>[5x]NEAVKTLDGWFCLHDFRSIDWAAWRELNPGNQELMLNELSHFLSDMEIT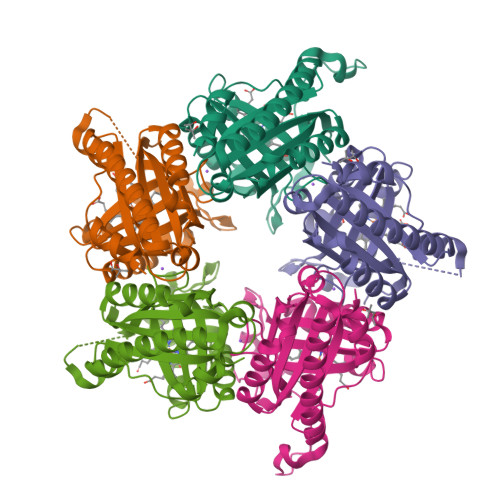KNIGEGEHTIYSILGQKADLVFFTLRDSLEALNEVENRFNKLAIADYLLPTYSYISVVELSNYLASHMAGGDDPYQNKGVRARLYPALPPKKHICFYPMSKKRDGADNWYMLPMEERQQLIRDHGLIGRSYAGKVQQIIGGSIGFDDYEWGVTLFSDDALEFKRIVTEMRFDEASARYAEFGSFFIGNLLLSEQLSKLFTI>MERTFLMIKPDAVQRNLIGEVISRIERKGLKLVGGKLMQVPMELAETHYGEHQGKPFYNDLISFITSAPVFAMVVEGEDAVNVSRHIIGSTNPSEASPGSIRGDLGLTVGRNIIHGSDSLESAEREINLW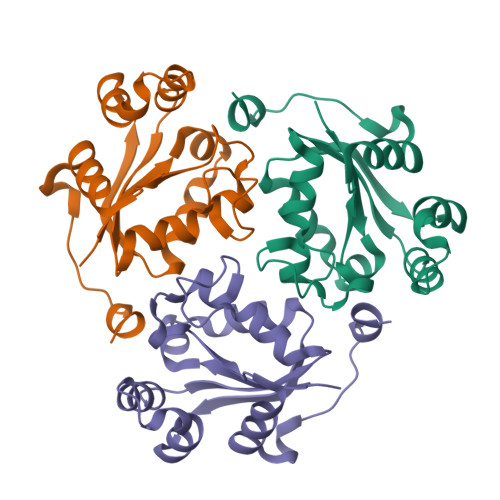FNENEITSYASPRDAWLYELEHHHHHH[6x]N-(4-oxo-1,4-dihydrocinnoline-3-carbonyl)glycine | C11 H9 N3 O4 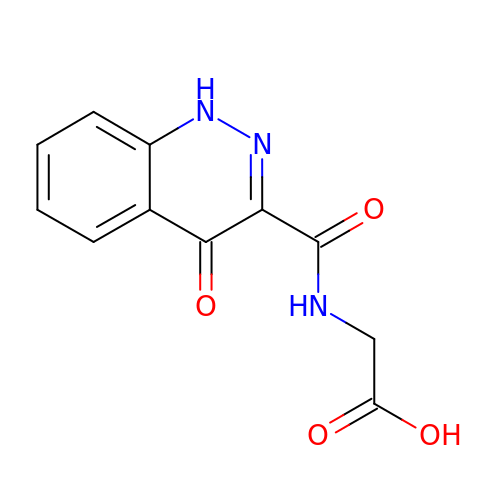| WSQQFPKJCSYPLX-UHFFFAOYSA-N> MVGAHQMKSEEQANMQLQQQAVLGLNWMQDSGEYKALAYQAYNAAKVAFDHAKVAKGKKKAVVADLDETMLDNSPYAGWQVQNNKPFDGKDWTRWVDARQSRAVPGAVEFNNYVNSHKGKVFYVTNRKDSSEKAGTIDDMKRLGFNGVEESAFYLKKDKSAKAARFAEIEKQGYEIVLYVGDNLDDFGNTVYGKLNADRRAFVDQNQGKFGKTFIMLPNANYGGWEGGLAEGYFKKDT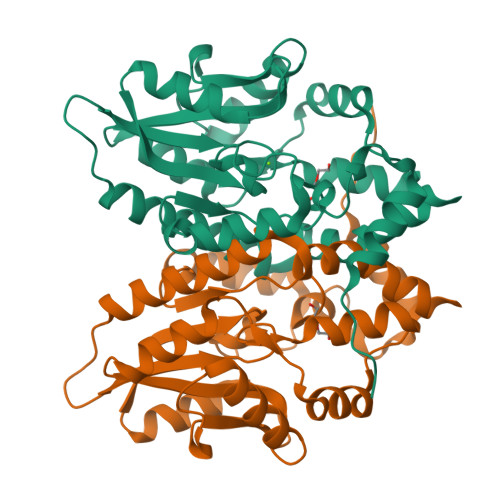QGQIKARLDAVQAWDGK> MLSDYEEFLRLEKARKIILEILNEKGRDALYDLSGLSGGFLIDEKDKALLNTYI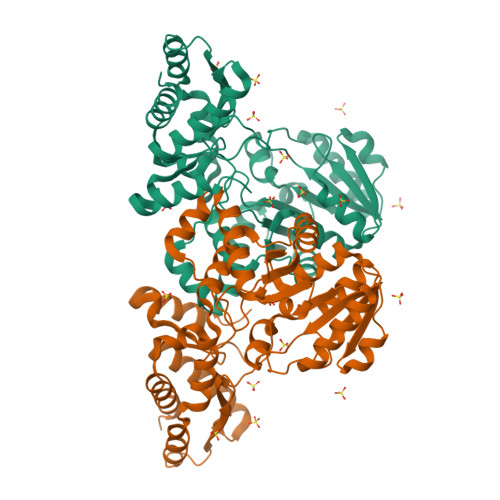GSSYFAEKVNEYGLKHLGGDENDKCVGFNRTSSAILATILALKPKKVIHYLPELPGHPSIERSCKIVNAKYFESDKVGEILNKIDKDTLVIITGSTMDLKVIELENFKKVINTAKNKEAIVFVDDASGARVRLLFNQPPALKLGADLVVTSTDKLMEGPRGGLLAGKKELVDKIYIEGTKFGLEAQPPLLAGIYRALKNFNLERIRKAFERAKNFDLSKIEKLNKELKAIDDNINIVYERTPTGFVIKRVYKDDTINIKKLIEIGFNLLKNYGIITITVAGMPGASKSLRIDLTSRDAERIDDNYIIKAIVESIKMAFKS>NTGIVSSFFTYTGPAHGTQWDEIDIEFLGKDTTKVQFNYYTNGVGGHEKVISLGFDASKGFHTYAFDWQPGYIKWYVDGVLKHTATANIPSTPGKIMMNLWNGTGVDDWLGSYNGANPLYAEYDWVKYTSNQTGGSFFEPFNSYNSGTWEKADGYSNGGVFNCTWRANNVNFTNDGKLKLGLTSSAYNKF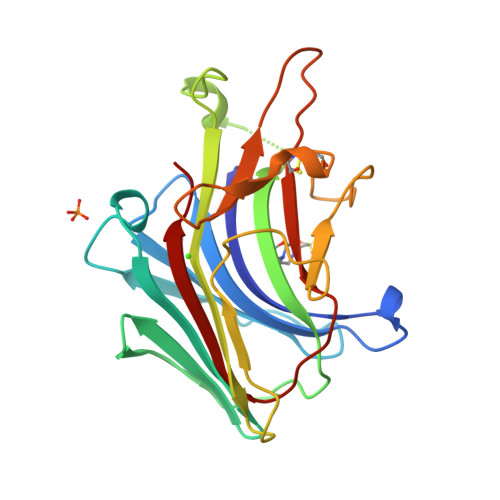DCAEYRSTNIYGYGLYEVSMKPAK[2x]> MSDSQTLVVKLGTSVLTGGSRRLNRAHIVELVRQCAQLHAAGHRIVIVTSGAIAAGREHLG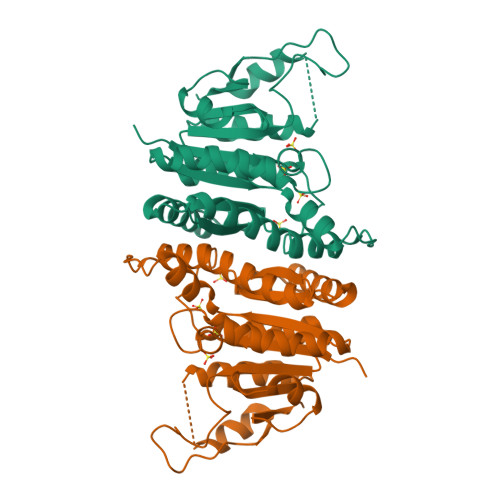YPELPATIASKQLLAAVGQSRLIQLWEQLFSIYGIHVGQMLLTRADMEDRERFLNARDTLRALLDNNVVPVINENDAVATAEIKVGDNDNLSALAAILAGADKLLLLTDQKGLYTADPRSNPQAELIKDVYGIDDALRAIAGDSVSGLGTGGMSTKLQAADVACRAGIDTIIAAGSKPGVIGDVMEGISVGTLFHAQA> GKRQWALEDFEIGRPLGKGKFG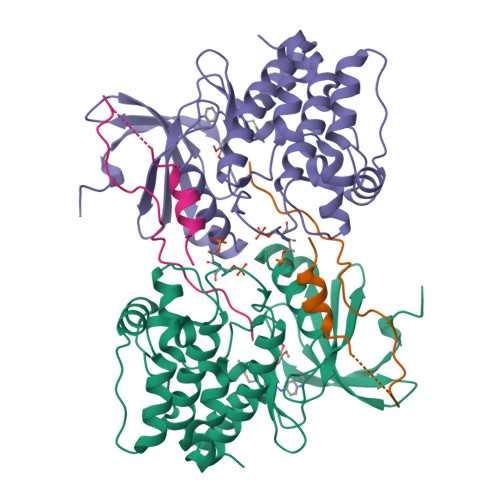NVYLAREKQSKFILALKVLFKAQLEKAGVEHQLRREVEIQSHLRHPNILRLYGYFHDATRVYLILEYAPLGTVYRELQKLSKFDEQRTATYITELANALSYCHSKRVIHRDIKPENLLLGSAGELKIADFGWSVHAPSSRRTTLCGTLDYLPPEMIEGRMHDEKVDLWSLGVLCYEFLVGKPPFEANTYQETYKRISRVEFTFPDFVTEGARDLISRLLKHNPSQRPMLREVLEHPWITANSSKPS;> GMSQVKSSYSYDAPSDFINFSSLDDEGDTQNIDSWFEEKANLEN>GSHMTQDCSFQHSPISSDFAVKIRELSDYLDQDYPVTVASNLQDEELCGGLWRLVLAQRWMERLKTVAGSKMQGLLER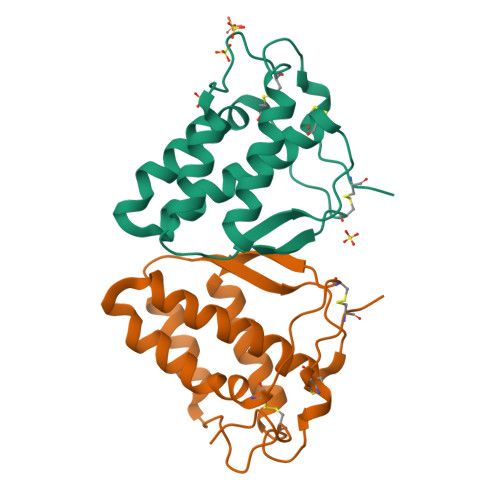VNTEIHFVTKCAFQPPPSCLRFVQTNISRLLQETSEQLVALKPWITRQNFSRCLELQCQP[2x]>[2x]MNPAAEAEFNILLATDSYKVTHYKQYPPNTSKVYSYFECREKKTENSKLRKVKYEETVFYGLQYILNKYLKGKVVTKEKIQEAKDVYKEHFQDDVFNEKGWNYILEKYDGHLPIEIKAVPEGFVIPRGNVLFTVENTDPECYWLTNWIETILVQSWYPITVATNSR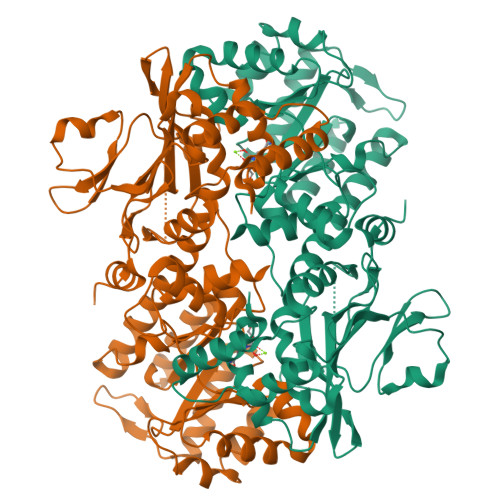EQKKILAKYLLETSGNLDGLEYKLHDFGYRGVSSQETAGIGASAHLVNFKGTDTVAGLALIKKYYGTKDPVPGYSVPAAEHSTITAWGKDHEKDAFEHIVTQFSSVPVSVVSDSYDIYNACEKIWGEDLRHLIVSRSTQAPLIIRPDSGNPLDTVLKVLEILGKKFPVTENSKGYKLLPPYLRVIQGDGVDINTLQEIVEGMKQKMWSIENIAFGSGGGLLQKLTRDLLNCSFKCSYVVTNGLGINVFKDPVADPNKRSKKGRLSLHRTPAGNFVTLEEGKGDLEEYGQDLLHTVFKNGKVTKSYSFDEIRKNAQLNI> GPASQDPTIFEERHLKYISQLGKGNFGSVELCRYDPLGDNTGALVAVKQLQHSGPDQQRDFQREIQILKALHSDFIVKYRGVSYGPGRQSLRLVMEYLPSGCLRDFLQRHRARLDASRLLLYSSQICKGMEYLGSRRCV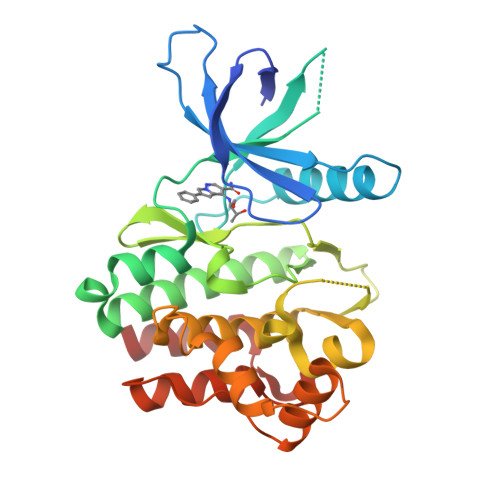HRDLAARNILVESEAHVKIADFGLAKLLPLDKDYYVVREPGQSPIFWYAPESLSDNIFSRQSDVWSFGVVLYELFTYCDKSCSPSAEFLRMMGSERDVPALSRLLELLEEGQRLPAPPACPAEVHELMKLCWAPSPQDRPSFSALGPQLDMLWS> GSMEYEWKPDEQGLQQILQLLKESQSPDTTIQRTVQQKLEQLNQYPDFNNYLIFVLTKLKSEDEPTRSLSGLILKNNVKAHFQNFPNGVTDFIKSECLNNIGDSSPLIRATVGILITTIASKGELQNWPDLLPKLCSLLDSEDYNTCEGAFGALQKICEDSAEILDSDVLDRPLNIMIPKFLQFFKHSSPKIRSHAVACVNQFIISRTQALMLHIDSFIENLFALAGDEEPEVRKNVCRALVMLLEVRMDRLLPHMHNIVEYMLQRTQDQDENVALEACEFWLTLAEQPICKDVLVRHLPKLIPVLVNGMKYSDIDIILLKGDVEEDETIPDSEQDIRGGSGGSGDTISDWNLRKCSAAALDVLANVYRDELLPHILPLLKELLFHHEWVVKESGILVLGAIAEGCMQGMIPYLPELIPHLIQCLSDKKALVRSITCWTLSRYAHWVVSQPPDTYLKPLMTELLKRILDSNKRVQEAACSAFATLEEEACTELVPYLAYILDTLVFAFSKYQHKNLLILYDAIGTLADSVGHHLNKPEYIQMLMPPLIQKWNMLKDEDKDLFPLLECLSSVATALQSGFLPYCEPVYQRCVNLVQKTLAQAMLNNAQPDQYEAPDKDFMIVALDLLSGLAEGLGGNIEQLVARSNILTLMYQCMQDKMPEVRQSSFALL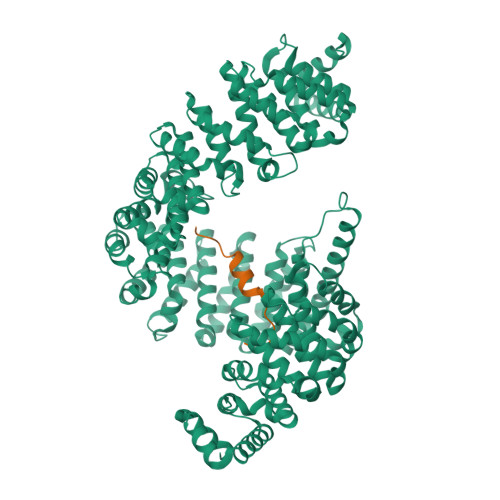GDLTKACFQHVKPCIADFMPILGTNLNPEFISVCNNATWAIGEISIQMGIEMQPYIPMVLHQLVEIINRPNTPKTLLENTAITIGRLGYVCPQEVAPMLQQFIRPWCTSLRNIRDNEEKDSAFRGICTMISVNPSGVIQDFIFFCDAVASWINPKDDLRDMFCKILHGFKNQVGDENWRRFSDQFPLPLKERLAAFYGV;> GGSRGGYDRGGYRGRGGDRGGFRGGRGGGDRGGFGPGKMDSRGEHRQDRRERLY4-[5-(4-FLUORO-PHENYL)-2-(4-METHANESULFINYL-PHENYL)-3H-IMIDAZOL-4-YL]-PYRIDINE | C21 H16 F 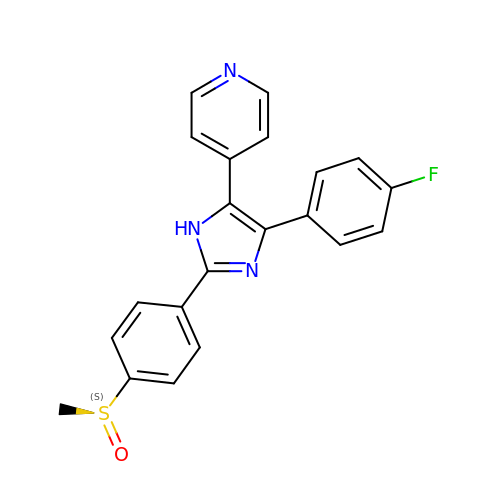N3 O S | CDMGBJANTYXAIV-MHZLTWQESA-N O-(2-ACETAMIDO-2-DEOXY D-GLUCOPYRANOSYLIDENE) AMINO-N-PHENYLCARBAMATE | C15 H19 N3 O7 | 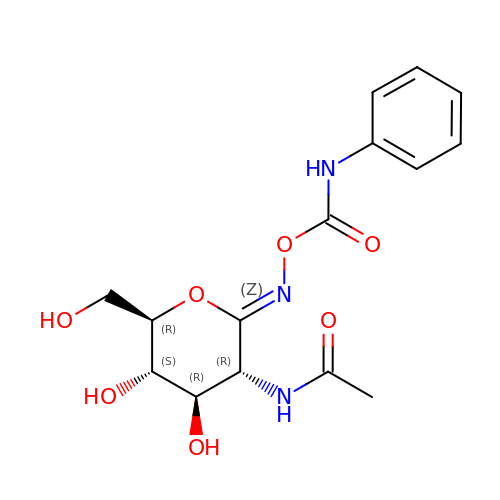PBLNJFVQMUMOJY-JXZOILRNSA-N> X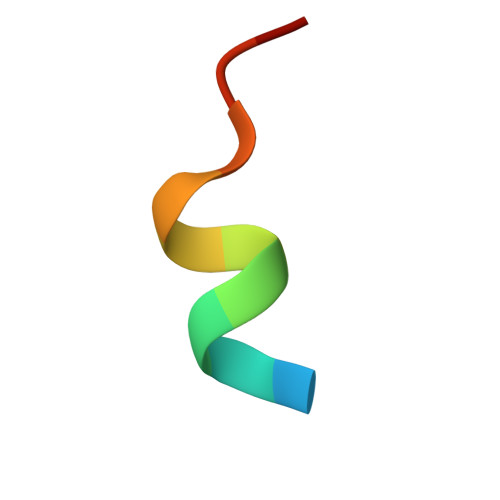CWEAWLLCETX3,5-diphenyl-2-(trifluoromethyl)-1~{H}-pyrazolo[1,5-a]pyrimidin-7-one | C19 H12 F3 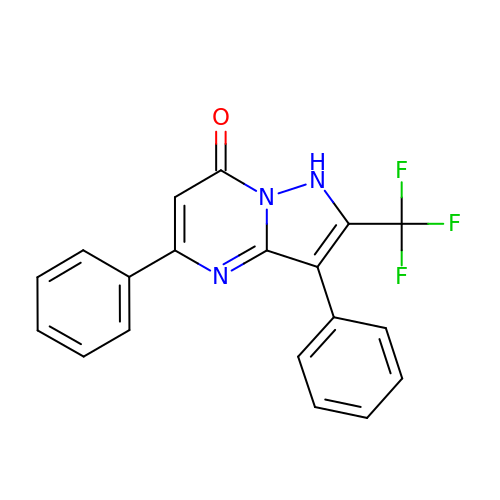N3 O | OOAHQJLYDSAULT-UHFFFAOYSA-N The human protein tyrosine phosphatase non-receptor type 3 (PTPN3) and the protein tyrosine phosphatase non-receptor type 4 (PTPN4) compose the NT5 type of non-transmembrane PTPs. These large modular proteins feature a N-terminal FERM (Band 4.1, Ezrin, Radixin, and Moesin) domain that is responsible for the localization of these enzymes to submembranous sites in the cell, a PDZ (PSD-95/Dlg/ZO-1) domain that allows specific binding to C-terminal recognition sequences in target proteins, and a C-terminal catalytic tyrosine phosphatase domain. The PDZ domain of PTPN3 (PTPN3-PDZ) has been identified as a target of the E6 PBM of HPV16 and 18. This PDZ-PBM interaction results in the ubiquitin-mediated proteasomal degradation of PTPN3.

The instability and tendency to oligomerize of PTPN3-PDZ made this construct unsuitable for crystallogenesis. To gain in stability and protein expression yield, we extended the N-terminal extremity of PTPN3-PDZ by 15-residues with its wild-type upstream sequence (PTPN3-PDZNext in Fig. 1). To investigate the molecular determinants of the interaction of PTPN3 with the HPV16 E6 protein, we solved the crystal structure of the complex formed by PTPN3-PDZNext and HPV16E6 PBM by molecular replacement at 2.19 Å resolution. PTPN3-PDZNext adopts a typical PDZ fold, with a β-sandwich comprising five β strands and two α helices. The PBM ligand binds in a hydrophobic cleft formed by the β2-strand, the α2-helix and the “GLGF” loop. HPV16E6 PBM binds to the PDZ domain as an anti-parallel extension of the β2-strand domain in a conventional mode. There is no electron density corresponding to the N-terminal extension of PTPN3-PDZNext in the crystal, which indicates a disordered region, in agreement with the NMR results that show an unfolded extension. A clear electron density map was seen for only the last seven C-terminal residues of HPV16E6 PBM (-TRRETQLCOOH) that are inserted into the binding groove. HPV16E6 PBM binding to PTPN3-PDZ is consistent with the binding mode observed for canonical class I PDZ domains, where L0 and T−2 are involved in key interactions with the PDZ domain. The hydroxyl group of threonine at position −2 forms a hydrogen bond with the Nε2 of the conserved histidine H572 from the α2-helix of PTPN3-PDZ. The side-chain carboxyl of E−3 forms a bifurcated H-bond with the hydroxyl of the conserved S538 (S545 for PTPN4) and N524 (N531 for PTPN4) amine group.

>GAMGSSTEDASQYYCDKNDNGDSYLVLIRITPDEDGKFGFNLKGGVDQKMPLVVSRINPESPADTCIPKLNEGDQIVLINGRDISEHTHDQVVMFIKASRESHSRELALVIRRR[6x];>[6x]RSSRTRRETQL>EPPKVEPPK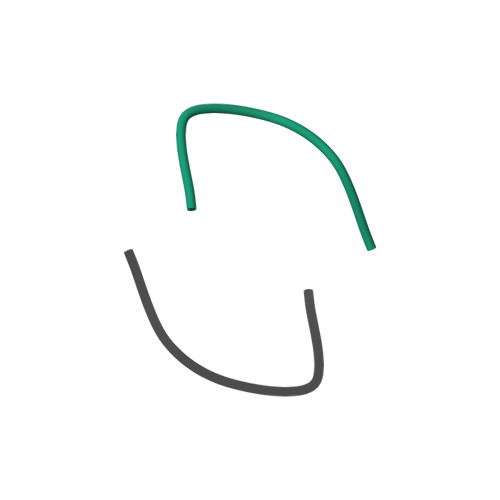V[2x]> MKIIKLYFESPVHFGEKRLSESKITFSADTLF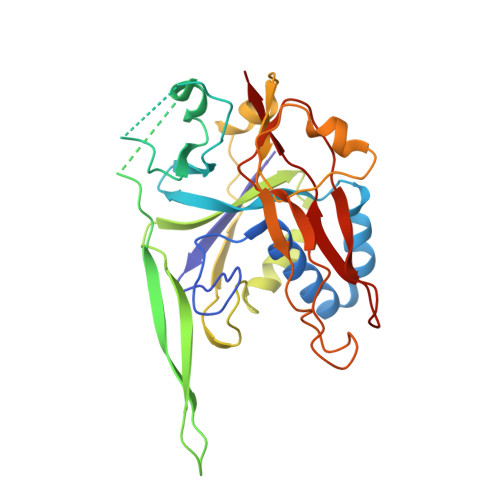SALMIEAVGLGKEDEFYQLASNNLVKFSDAFPFIDQYYYIPKPMFNLKLEKEDENPSKAFKKLLYVPIDSLEDYLSGGLDAYFERESFNLGKLALSEKVQQHDFKDSEPYNVGTFTFKENTGLYVLIEQTHPLLEELLENLQYSGIGGKRNSGYGKFKFEILEDSDIEDLFSAKGNRKILLSGALPKDAELEQALKNASYLLERRGGFVQSDTYATNLVKKQDLYVFKSGSTFENSFDGDIYQVGKKGNHPVYKYAKSFFLEVS(4S,5R)-2-(4-tert-butyl-2-ethoxyphenyl)-4,5-bis(4-chlorophenyl)-4,5-dimethyl-4,5-dihydro-1H-imidazole | C29 H32 Cl2 N2 O | 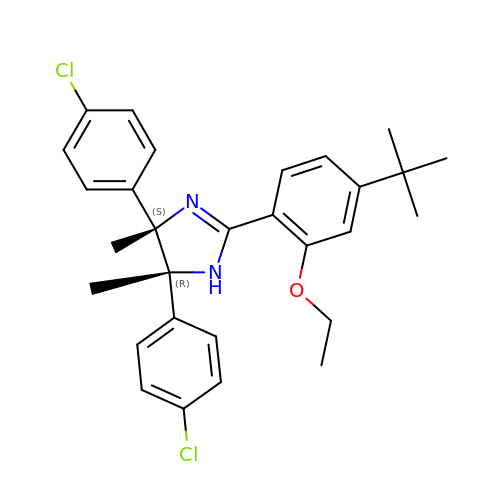OOVOROVEJRZNDO-ISILISOKSA-N>[2x]MQARKLAVDGAIEFTPRVFADDRGLLILPYQEEAFVEAHGGPLFRVAQTIHSMSKRGVVRGIHYTVTPPGTAKYVYCARGKAMDIVIDIRVGSPTFGQWDSVLMDQQDPRAV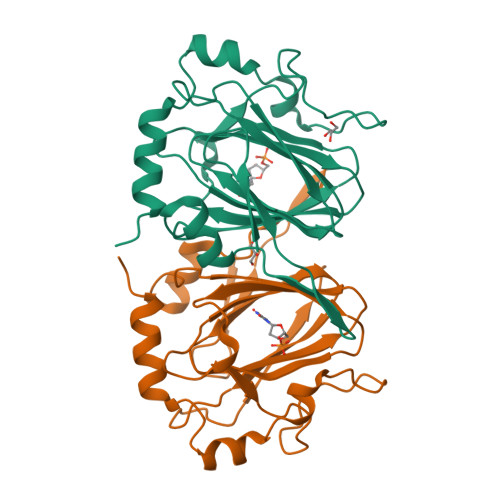YLPVGVGHAFVALEDDTVMSYMLSRSYVTQDELALSALDPALGLPIDIGVEPIVSDRDRVAITLAEAQRQGLLPDYTTSQEIERRLTAVPVST> MSKTVEDRAAQRAKGPATVLAIGTATPANVVYQTDYPDYYFRVTKSEHMTKLKNKFQRMCDRSTIKKRYMVLTEELLEKNLSLCTYMEPSLDARQDILVPEVPKLGKEAADEAIAEWGRPKSEITHLIFCTTCGVDMPGADYQLTKLLGLRSSVRRTMLYQQGXFGGGTVLRLAKDLAEN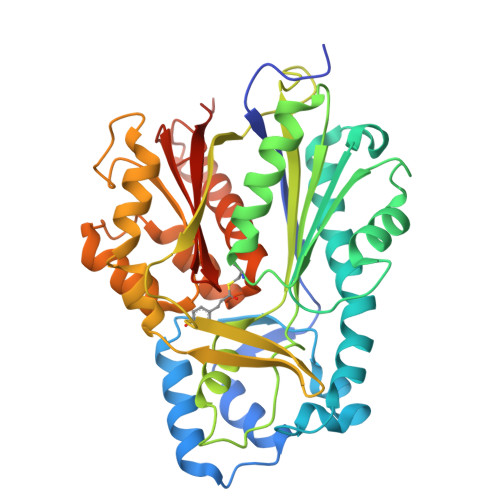NAGARVLVVCSEITTAVNFRGPSDTHLDLLVGLALFGDGAAAVIVGADPDPTLERPLFQIVSGAQTILPDSEGAINGHLREVGLTIRLLKDVPGLVSMNIEKCLMEAFAPMGIHDWNSIFWIAHPGGPTILDQVEAKLGLKEEKLKSTRAVLREYGNMSSACVLFILDEVRKRSMEEGKTTTGEGFDWGVLFGFGPGFTVETVVLHSMPIPKADEGR> QQKILENIRGIGTNTMTIFNGNGFGDRRSRHIQNLKISDANTLSKQSYIQSVTPNTSSSGILVVGNKSFTSANLYGIGEQYFDVEGLKLKQGRLLTEDDVDQSNQVVVLDESAKKAIFANENPLGKTVIFNKRPFRVIGVVSDQQLGGFPGNS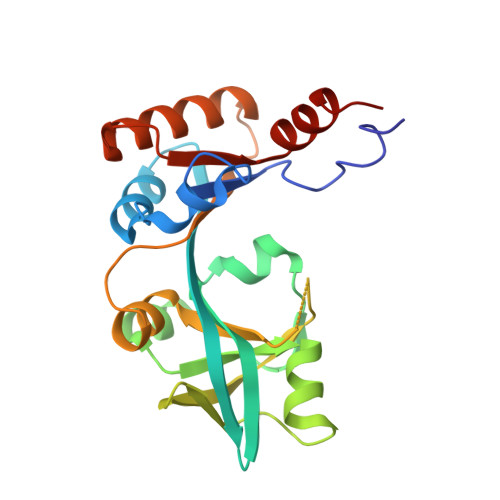LNLYSPYSTVLNKITGGSRIGSITVKISDDVNSTVAEKSLTELLKSLHGKKDFFIMNSDTIKQTIENTTGTMK> GPGSEFDTRH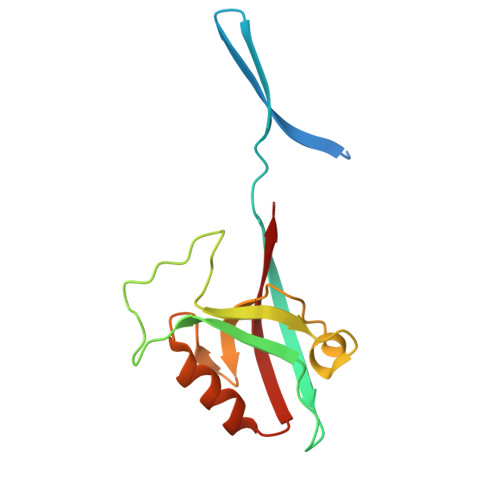ETREDRTKRLFRHYTVGSYDSLTSHSDYVIDDKVAILQKRDHEGFGFVLRGAKAETPIEEFTPTPAFPALQYLESVDVEGVAWRAGLRTGDFLIEVNGVNVVKVGHKQVVGLIRQGGNRLVMKVVSVTR5'-O-[N-(3-Indolepropionic acid)sulfamoyl] N2-methyl-2-aminoethenoadenosine | C24 H26 N8 O7 S | 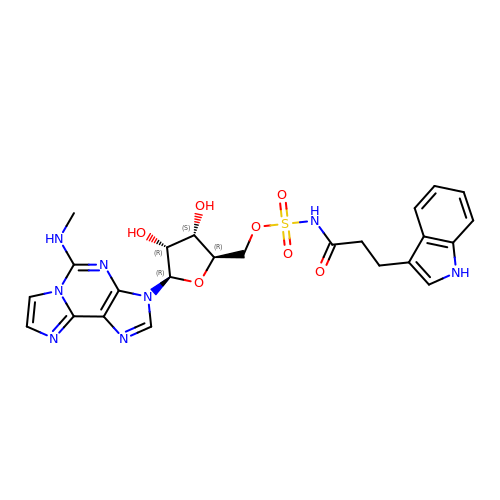MCGJNWYQNXMIEN-UGTJMOTHSA-N> GPLGSEKIEKDNAFAFDLLQTTRKHVTEANVFISPLSVSMALNMTLNGAAGVTADEMKTALRETGYTMEDINEYSHSLREALLKVDPSTTIGMANSIWYKQGELVKEPFILANRTHYDAEVK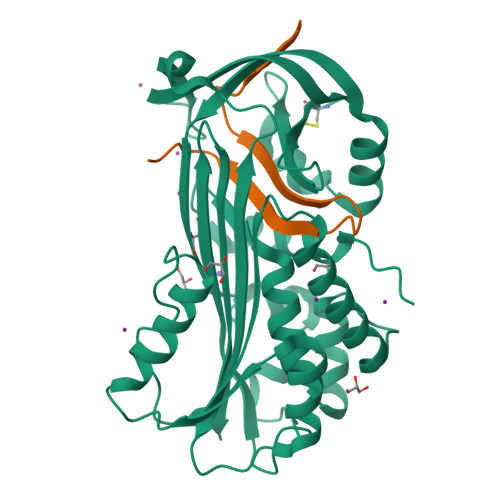AVDFSSPATLPAINGWCAQKTNDKITKILDYIPGNAFMYLINAVYFKGIWVTQFKKSDTKRAPFRKADGTTQEVNMMAQKSTFGYTTDECCQYLEMDYGNKAFSMIVMLPNEGQTTRDVIEQLDNKHWSMIIKGIRPTQVSLRMPRFKTECKYGLEKKILPEMGMNVPFTETADFPGITDAAIFISRVIHKTFVQVDEEGTEAAAVTAVEMVKT;> SSPSTTPINFHINKPFVFAIREKSTGVILFIGEIGEVKE> SENLYFQG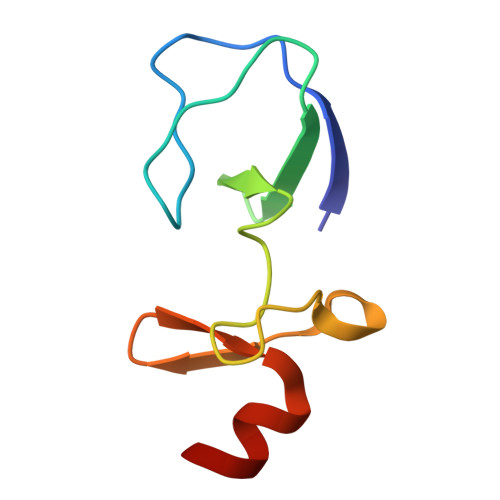SASATCERCKGGFAPAEKIVNSNGELYHEQCFVCAQCFQQFPEGLFYEFEGRKYCEHDFQMLFA>MASKEIKPIENSIVKEIIVKEGESVRKGDVLLKLTALGAEADTLKTQSSLLQTRLEQTRYQIL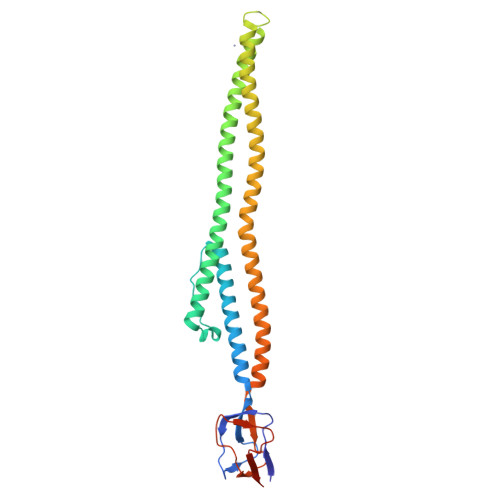SRSIELNKLPELKLPDEPYFQNVSEEEVLRLTSLIKEQFSTWQNQKYQKELNLDKKRAERLTILARINRYENLSRVEKSRLDDFRSLLHKQAIAKHAVLEQENKYVEAANELRVYKSQLEQIESEILSAKEEYQLVTRLFKNEILDKLRQTTDNIELLTLELEKNEERQQASVIRAPVSGKVQQLKVHTEGGVVTTAETLMVIVPEDDTLEVTALV[4x]Enzymes of the vanillyl alcohol oxidase/p-cresol methyl hydroxylase (VAO/PCMH) superfamily are found across all kingdoms where they perform a range of metabolic functions. These flavoproteins share a conserved FAD-binding domain and a more variable substrate-binding domain that enables interactions with a range of substrates. One of these, the 4-phenol oxidases/dehydrogenases, catalyzes the oxidation of para-substituted phenolic compounds. A fundamental distinction is that the oxidases efficiently react with oxygen producing hydrogen peroxide whereas the dehydrogenases hardly react with oxygen and typically employ other proteins, such as cytochrome c, as acceptors.

The enzyme from Novosphingobium sp. was of particular interest because it was predicted to lack a covalent flavin and to feature an unusual Val/Thr pair around the flavin N5 site, beside sharing 43% and 36% sequence identity with VAD and VAO, respectively. The same properties were exhibited also by the T181D variant mutant, targeting the threonine residue that is typically an aspartate in the known sequence-related oxidases. The enzyme was therefore named as nsVAO, although we cannot exclude that it might use an endogenous cytochrome rather than oxygen as physiological substrate. Its crystal structure confirms that FAD is non-covalently bound, supporting the notion that removal of the covalent flavin linkage does not drastically affect the properties of VAO/PCMH enzymes. The protein exhibits a narrow tunnel leading of the flavin re side where Val181, homologous to Pro151 of VAD, is in direct contact with the N5 atom.

>[2x]ADFAGAMKAFRGVVGAEWVFGDEEAVVPWSKTYIPDPAHQYKPVGAVCPQSVEEVQEIVRIANTYKQPLWTVSTGKNMGYGMTAPATPGQVVLDLKRMNRILEVDADLGTCLLEPGVTYQQLKDYLEEHKIPLWIDVPDVGPIASPVGNTLDRGVGYTPYGEHFMFQCGMEVCLPDGRLMRTGMGSIKGSTAWQAFKWGYGPYLDGLFTQSNFGIVTKMGLWLMPKPPVYKPFMVRHANMEDVPKIIEAMRPLRVSNLVANCNLMMSASYQLAMFKRRNEIVPDGAPLDEASLKKAASANGLGMWNTYFALYGTEQTVAGVEPIIRATLTASGGEVLTAAEMEGNPWFHHHQTLMQGGLNLDEVGLLRWRGAGGGLAWFAPVAAARGVEAERQTALAKEIVEKHGFDYTAAYAIGWRDLHHIIALLFDKADPTQEQKADACYRELVTRFGAQGWASYRTGVNSMDLVAQQYGEVNRDFNRTLKRAIDPNGILSPGKSGIHP> SPMAVEEVIEMQGLSLDPTSHRVMAGEEPLEMGPTEFKLLHFFMTHPERVYSREQLL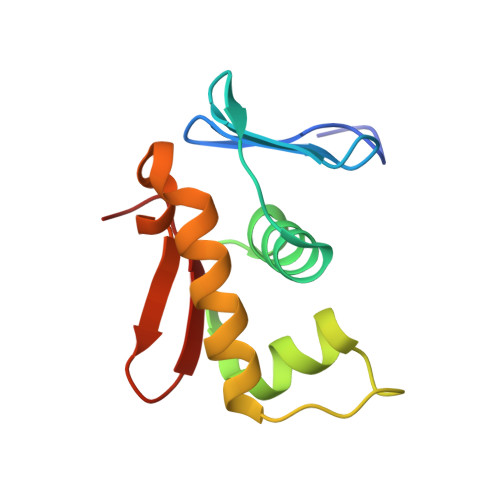NHVWGTNVYVEDRTVDVHIRRLRKALEPGGHDRMVQTVRGTGYRFSTRF2-chloro-6-(4-{[(3,4-dichloro-5-methyl-1H-pyrrol-2-yl)carbonyl]amino}piperidin-1-yl)pyridine-4-carboxamide | 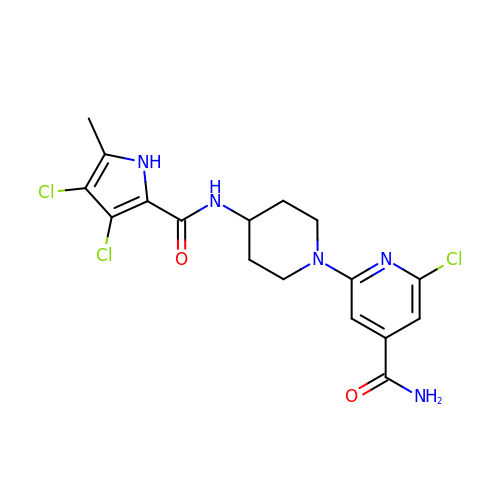C17 H18 Cl3 N5 O2 | DDZQOAWVENUEIU-UHFFFAOYSA-N> 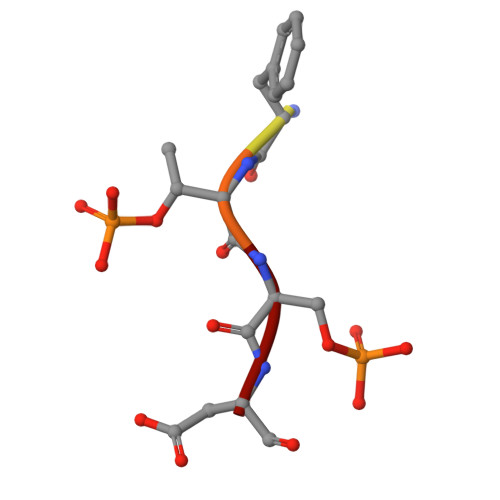MDFTSD The PBP family is responsible for the synthesis and cross-linking of peptidoglycan, the major component in the bacterial cell wall. The cell wall plays a pivotal role in controlling the shape and integrity of the cell and inhibition of the PBPs leads to cell lysis due to turgor pressure. The penicillin-binding domain contains a catalytic serine residue, which is vital for its function and a useful target for inhibition. Due to their essential role in cell division and elongation, PBPs are attractive targets for antibiotics with many β-lactam antibiotics developed for this purpose.

Due to this imminent need for new antibiotic leads, our DOS library was screened against P. aeruginosa PBP3 using the XChem platform. The core enol lactone scaffold was found to react with Ser294, the catalytic residue found within the conserved SXXK motif of the β-lactam binding pocket. Upon incubation of the compound with the crystals, resulting electron density maps suggested a linear bound compound, which was hypothesised to result from lactone ring-opening followed by enol tautomerization to afford the linear ketone derivative. In addition to the covalent bond, hydrogen bonding interactions were observed with neighbouring residues Asn351, Ser349 and Thr487. Considering these findings, it was proposed that the identified hit could be rapidly diversified through four primary vectors to comprehensively probe the PBP3 binding pocket. The 10 elaborated analogues were then screened using X-ray crystallography to validate the initial hit and observe the effects of vector derivatisation on the PBP3 binding preference. All compounds except for 8–11 were identified as PBP3 binders using this method. This preliminary data proved to be extremely useful in validating this hit with all analogues covalently binding to Ser294 in a similar fashion to that of 1, whilst the specificity for the 5-membered lactone and terminal alkene could be inferred. The hit identified against PBP3 binds through a covalent mechanism, exemplifying the utility of our library towards the discovery of novel covalent ligands, in addition to reversible binders. Indeed, similar electrophilic fragments have been demonstrated to have enhanced utility in probe development due to their high duration of action and potency.

> GPGYQDPARSVRHIAIPAHRGLITDRNGEPLAVSTPVTTLWANPKELMTAKERWPQLAAALGQDTKLFADRIEQNAEREFIYLVRGLTPEQGEGVIALKVPGVYSIEEFRRFYPAGEVVAHAVGFTDVDDRGREGIELAFDEWLAGVPGKRQVLKDRRGRVIKDVQVTKNAKPGKTLALSIDLRLQYLAHRELRNALLENGAKAGSLVIMDVKTGEILAMTNQPTYNPNNRRNLQPAAMRNRAMIDVFEPGSTVKPFSMSAALASGRWKPSDIVDVYPGTLQIGRYTIRDVSRNSRQLDLTGILIKSSNVGISKIAFDIGAESIYSVMQQVGLGQDTGLGFPGERVGNLPNHRKWPKAETATLAYGYGLSVTAIQLAHAYAALANDGKSVPLSMTRVDRVPDGVQVISPEVASTVQGMLQQVVEAQGGVFRAQVPGYHAAGKSGTARKVSVGTKGYRENAYRSLFAGFAPATDPRIAMVVVIDEPSKAGYFGGLVSAPVFSKVMAGALRLMNVPPDNLPTA>[2x]GPLGSGLFRSKHTTSQKNFYDNLTSTLLRLSTDKIGAIIAIE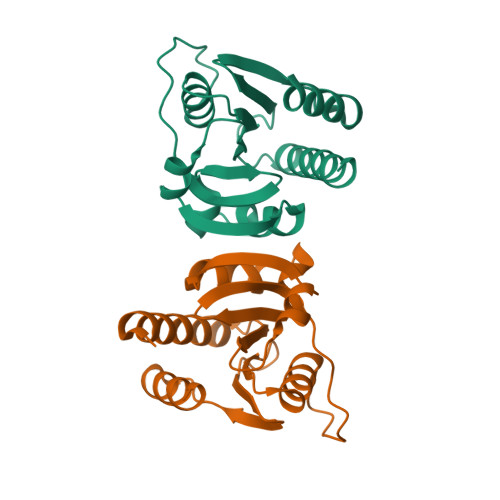NQDSLESYVNIGYRVTSDFSPELLVTIFYNKQSPLHDGAVIVRDYQIVSVSSYFPMTRQLIDVSYGSRHRSALGLTEKCDAIVFIVSETTGKISVAVRGVIKTLSSNSDRLQDQIIHYLTVKPG> SEDDLTKVLNYTKQRQTEPNPEYYGVAKKKNIIKIHLESFQTFLINKKVNGKEVTPFLNKLSSGKEQFTYFPNFFHQTGQGKTSDSEFTMDNSLYGLPQGSAFSLKGDNTYQSLPAILDQKQGYKSDVMHGDYKTFWNRDQVYKHFGIDKFYDATYYDMSDKNVVNLGLKDKIFFKDSANYQAKMKSPFYSHLITLTNHYPFTLDEKDATIEKSNTGDATVDGYIQTARYLDEALEEYINDLKKKGLYDNSVIMIYGDHYGISENHNNAMEKLLGEKIT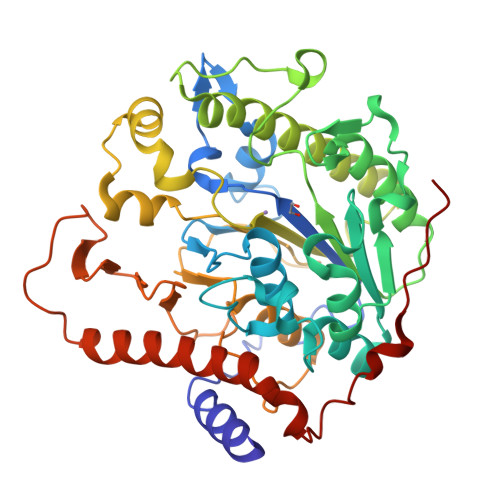PAKFTDLNRTGFWIKIPGKSGGINNEYAGQVDVMPTILHLAGIDTKNYLMFGTDLFSKGHNQVVPFRNGDFITKDYKYVNGKIYSNKNNELITTQPADFEKNKKQVEKDLEMSDNVLNGDLFRFYKNPDFKKVNPSKYKYETGPK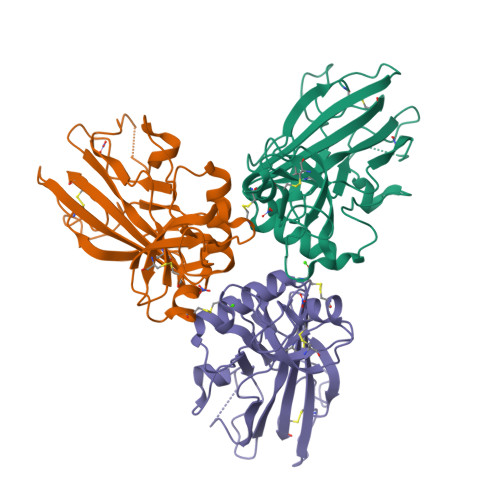>[3x]ETGHHHHHHSADEPMDFKINTDEIMTSLKSVNGQIESLISPDGSRKNPARNCRDLKFCHPELKSGEYWVDPNQGCKLDAIKVFCNMETGETCISANPLNVPRKHWWTDSSAEKKHVWFGESMDGGFQFSYGNPELPEDVLDVQLAFLRLLSSRASQQITYHCKNSIAYMDQASGNVKKALKLMGSNEGEFKAEGNSKFTYTVLEDGCTKHTGEWSKTVFEYRTRKAVRLPIVDIAPYDIGGPDQEFGVDVGPVCFL3-(1-benzothiophen-3-yl)-L-alanine | C11 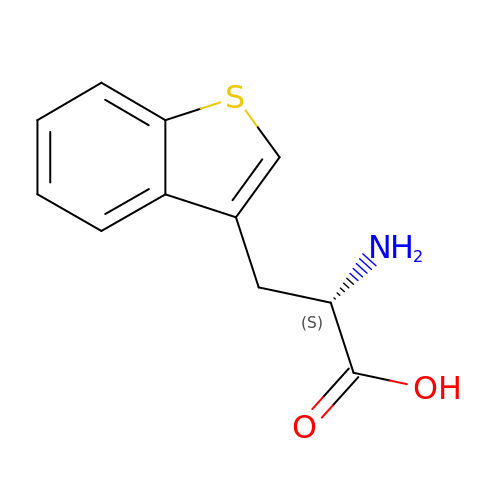H11 N O2 S | GAUUPDQWKHTCAX-VIFPVBQESA-N> GATVAPSSRRDFTFDLYRALASAAPSQNIFFSPVSISMSLAMLSLGAGSSTKMQILEGLGLNLQKSSEKELHRGFQQLLQELNQPRDGFQLSLGNALFTDLVVDLQDTFVSAMKTLYLADTFPTNFRDSAGAMKQINDYVAKQTKGKIVDLLKNLDSNAVVIMVNYIFFKAKWETSFNHKGTQEQDFYVTSETVVRVPMMSREDQYHYLLDRNLSCRVVGVPYQGNATALFILPSEGKMQQVENGLSEKTLRKWLKMFKKRQLE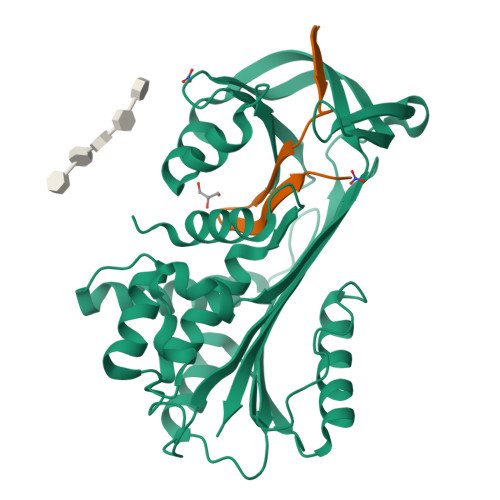LYLPKFSIEGSYQLEKVLPSLGISNVFTSHADLSGISNHSNIQVSEMVHKAVVEVDESGTRAAAATGTIFTF;> RSQRLVFNRPFLMFIVDNNILFLGKVNRP> GENLYFQGMRCIGMSNRDFVEGVSGGSWVDIVLEHGSCVTTMAKNKPTLDFELIKTEAKQPATLRKYCIEAKLTNTTTESRCPTQGEPSLNEEQDKRFVCKHSMVDRGWGNGCGLFGKGGIVTCAMFRC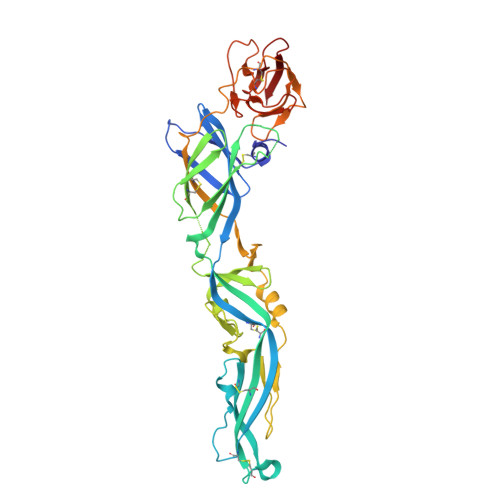KKNMEGKVVQPENLEYTIVITPHSGEEHAVGNDTGKHGKEIKITPQSSITEAELTGYGTVTMECSPRTGLDFNEMVLLQMENKAWLVHRQWFLDLPLPWLPGADTQGSNWIQKETLVTFKNPHAKKQDVVVLGSQEGAMHTALTGATEIQMSSGNLLFTGHLKCRLRMDKLQLKGMSYSMCTGKFKVVKEIAETQHGTIVIRVQYEGDGSPCKIPFEIMDLEKRHVLGRLITVNPIVTEKDSPVNIEAEPPFGDSYIIIGVEPGQLKLNWFKK>MDHLPIFCQLRDRDCLIVGGGDVAERKARLLLEAGARLTVNALTFIPQFTVWANEGMLTLVEGPFDETLLDSCWLAIAATDDDTVNQRVSDAAESRRIFCNVVDAPKAASFIMPSIIDRSPLMVAVSAGGTSGVLARLLREKLESLLPQHLGQVARYAGQLRARVKKQFATMGERRRFWEKFFVNDRLAQSLANADEKAVNATTERLFSEPLDHRGEVVLVGAGPGDAGLLTLKGLQQIQQADIVVYDRLVSDDIMNLVRRDADRVFVGKRAGYHCVPQEEINQILLREAQKGKRVVRLKGGDPFIFGRGGEELETLCHAGIPFSVVPGITAASGCSAYSGIPLTHRDYAQSVRLVTGHLKTGGELDWENLAAEKQTLVFYM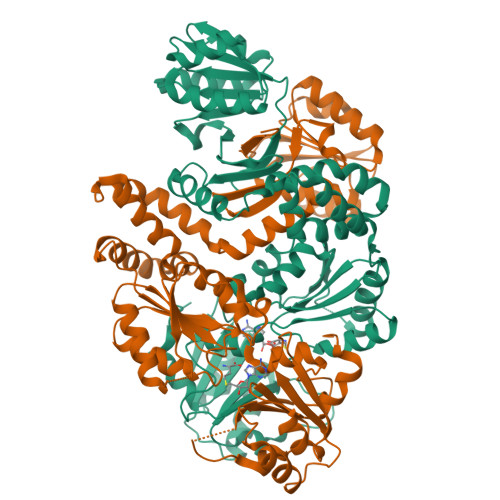GLNQAATIQEKLIAFGMQADMPVALVENGTSVKQRVVHGVLTQLGELAQQVESPALIIVGRVVALRDKLNWFSNH[2x]>MARIAQHISELIGGTPLVRLNSVVPDGAGTVAAKVEYLNPGGSSKDRIAVKMIEAAEASGQLKPGGTIVEPTSGNTGVGLALVAQRRGYKCVFVCPDKVSEDKRNVLIAYGAEVVVCPTAVPPHDPASYYSVSDRLVRDIDGAWKPDQYANPEGPASHYVTTGPEIWADTEGKVTHFVAGIGTGGTITGAGRYLKEVSGGRVRIVGADPEGSVYSGGAGRPYLVEGVGEDFWPAAYDPSVPDEIIAVSDSDSFDMTRRLAREEAMLVGGSCGMAVVAALKVAEEAGPDALIVVLLPDGGRGYMSKIFNDAWMSSYGFLRSRLDGSTEQSTVGDVLRRKSGALPALVHTHPSETVRDAIGILREYGVSQMPVVGAEPPVMAGEVAGSVSERELLSAVFEGRAKLADAVSAHMSPPLRMIGAGELVSAAGKALRDWDALMVVEEGKPVGVITRYDLLGFLSEGAGRRKLAAALEHHHHHH[4x]

Using a combination of biochemistry and cryo–electron microscopy, we characterized the first enzyme of the transsulfuration pathway, cystathionine β-synthase (MtbCbs) in Mtb. We demonstrated that MtbCbs is a heme-less, pyridoxal-5′-phosphate–containing enzyme, allosterically activated by S-adenosylmethionine (SAM). The rectangular-shaped 3D structure of the tetrameric MtbCbs contains an N-terminal catalytic core region (7 to 296 residues), C-terminal Bateman module (329 to 464 residues), and a connecting linker between the catalytic core and the Bateman module (297 to 328 residues). In this study, we resolved the full-length structure of MtbCbs in its native, activated, and substrate-bound conformations.

As the substrate channel expands after SAM treatment, our next target was to observe the changes after SAM and substrate Ser incubation. However, substrate-treated cryo-EM map demonstrated that the interaction between K44 and PLP is disrupted after Ser treatment, followed by the formation of external aldimine/aminoacrylate at the active site, which indicates association of Ser with PLP, in agreement with previous reports, which is strongly supported by our structural studies. (G) Serine binding converts protonated internal aldimine form to external aldimine and aminoacrylate intermediates. Furthermore, we were able to capture the formation of the external aldimine/aminoacrylate in presence of the substrate Ser at the enzyme’s active site. However, our study cannot distinguish between these two intermediates (external aldimine and aminoacrylate) from this resolution structure.>GPGSMAFLLHQARFFTTVNHLRDLPPTVQPEIAFAGRSNAGKSTAINVLCNQKRLAFASKTPGRTQHINYFSVGPAAEPVAHLVDLPGYGYAEVPGAAKAHWEQLLSSYLQTRPQLCGMILMMDARRPLTELDRRMIEWFAPTGKPIHSLLTKCDKLTRQESINALRATQKSLDAYRDAG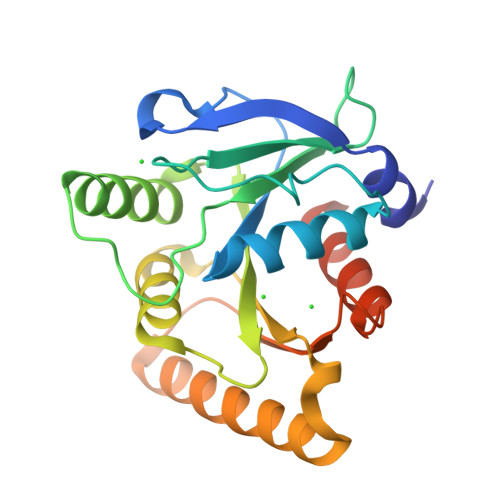YAGKLTVQLFSALKRTGLDDAHALIESWLRPAAADEDHAAVAE[2x]3-(3,5-dimethylphenyl)-2,1-benzoxazole-5-carboxylic 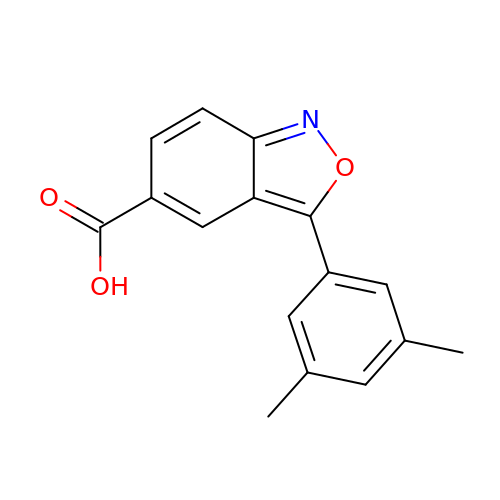acid | C16 H13 N O3 | QBHYQWOHSDLSMR-UHFFFAOYSA-N>GASPSAQELKEQGNRLFVGRKYPEAAACYGRAITRNPLVAVYYTNRALCYLKMQQHEQALADCRRALELDGQSVKAHFFLGQCQLEMESYDEAIANLQRAYSLAKEQRLNFGDDIPSALRIAKKKRWNSIEERR[2x];>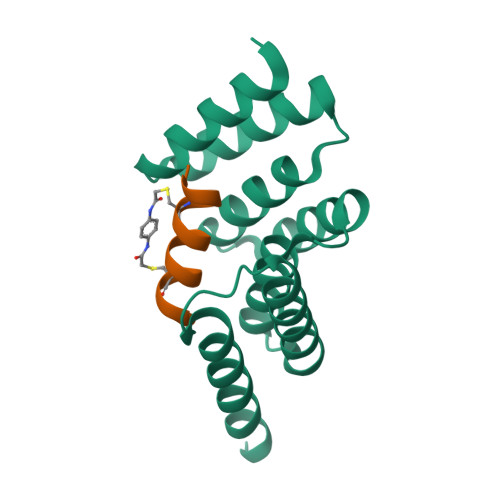[2x]XPLDLCYWASLHCIVSX The eukaryotic Structural Maintenance of Chromosomes (SMC) family includes the protein complexes cohesin, condensin and Smc5/6. The Smc5/6 complex plays an essential role in the resolution of recombination intermediates formed during mitosis or meiosis, or as a result of the cellular response to replication stress. The Smc5/6 complex has roles in the processes of DNA replication and DNA damage repair; the complex acting to suppress / prevent formation of inappropriate structures that can form during homologous recombination-mediated rescue of replication forks that have stalled (or collapsed) on encountering replication ‘road-blocks’ or obstacles. As well as containing subunits that provide both ubiquitin and SUMO E3-ligase activity (through Nse1 and Nse2 respectively), Smc5/6 is further differentiated from the cohesin and condensin complexes by the fact that the two non-SMC proteins (Nse1 and Nse3) that bind to its kleisin subunit (Nse4) belong to the ‘KITE’ family (kleisin-interacting tandem winged-helix element; 15) rather than the distinct and structurally unrelated ‘HAWK’ family (HEAT proteins associated with kleisins; 16).

Here, we report the cryogenic EM (cryo-EM) structure of the six-subunit budding yeast Smc5/6 holo-complex, reconstituted from recombinant proteins expressed in insect cells – providing both an architectural overview of the entire complex and an understanding of how the Nse1/3/4 subcomplex binds to the hetero-dimeric SMC protein core. Here, we have determined a cryo-EM structure for the budding yeast Smc5/6 ‘holo-complex’, in its apo or non-liganded form. Our study serves to confirm the overall architecture of the complex, plus provide details of how and where the Nse1/Nse3/Nse4 KITE-kleisin subcomplex interacts with the Smc5/Smc6/Nse2 core. Additional experiments also reveal the presence of a crucial interface formed between the head domain of Smc5 and Nse1, which utilises the equivalent of the ‘W-loop’ or ‘F-loop’ found in Smc4 and Smc1 respectively. Notably, mutations that alter the surface-charge profile of the region of Nse1 which accepts the Smc5-loop, lead to a slow-growth phenotype and a global reduction in the chromatin-associated fraction of the Smc5/6 complex, as judged by single molecule localisation microscopy experiments in live yeast. Taken together, our data uncover an unanticipated degree of functional equivalence between KITE and HAWK accessory subunits.

> MTSLIDLGRYVERTHHGEDTEPRSKRVKIAKPDLSSFQPGSIIKIRLQDFVTYTLTEFNLSPSLNMIIGPNGSGKSTFVCAVCLGLAGKPEYIGRSKKVEDFIKNGQDVSKIEITLKNSPNVTDIEYIDARDETIKITRIITRSKRRSDYLINDYQVSESVVKTLVAQLNIQLDNLCQFLSQERVEEFARLKSVKLLVETIRSIDASLLDVLDELRELQGNEQSLQKDLDFKKAKIVHLRQESDKLRKSVESLRDFQNKKGEIELHSQLLPYVKVKDHKEKLNIYKEEYERAKANLRAILKDKKPFANTKKTLENQVEELTEKCSLKTDEFLKAKEKINEIFEKLNTIRDEVIKKKNQNEYYRGRTKKLQATIISTKEDFLRSQEILAQTHLPEKSVFEDIDIKRKEIINKEGEIRDLISEIDAKANAINHEMRSIQRQAESKTKSLTTTDKIGILNQDQDLKEVRDAVLMVREHPEMKDKILEPPIMTVSAINAQFAAYLAQCVDYNTSKALTVVDSDSYKLFANPILDKFKVNLRELSSADTTPPVPAETVRDLGFEGYLSDFITGDKRVMKMLCQTSKIHTIPVSRRELTPAQIKKLITPRPNGKILFKRIIHGNRLVDIKQSAYGSKQVFPTDVSIKQTNFYQGSIMSNEQKIRIENEIINLKNEYNDRKSTLDALSNQKSGYRHELSELASKNDDINREAHQLNEIRKKYTMRKSTIETLREKLDQLKREARKDVSQKIKDIDDQIQQLLLKQRHLLSKMASSMKSLKNCQKELISTQILQFEAQNMDVSMNDVIGFFNEREADLKSQYEDKKKFVKEMRDTPEFQSWMREIRSYDQDTKEKLNKVAEKYEEEGNFNLSFVQDVLDKLESEIAMVNHDESAVTILDQVTAELRELEHTVPQQSKDLETIKAKLKEDHAVLEPKLDDIVSKISARFARLFNNVGSAGAVRLEKPKDYAEWKIEIMVKFRDNAPLKKLDSHTQSGGERAVSTVLYMIALQEFTSAPFRVVDQINQGMDSRNERIVHKAMVENACAENTSQYFLITPKLLTGLHYHEKMRIHCVMAGSWIPNPSEDPKMIHFGETSNYSFD;> MISTTISGKRPIEQVDDELLSLTAQQENEEQQQQRKRRRHQFAPMTQFNSNTLDEDSGFRSSSDVATADQDNFLEESPSGYIKKVILRNFMCHEHFELELGSRLNFIVGNNGSGKSAILTAITIGLGAKASETNRGSSLKDLIREGCYSAKIILHLDNSKYGAYQQGIFGNEIIVERIIKRDGPASFSLRSENGKEISNKKKDIQTVVDYFSVPVSNPMCFLSQDAARSFLTASTSQDKYSHFMKGTLLQEITENLLYASAIHDSAQENMALHLENLKSLKAEYEDAKKLLRELNQTSDLNERKMLLQAKSLWIDVAHNTDACKNLENEISGIQQKVDEVTEKIRNRQEKIERYTSDGTTIEAQIDAKVIYVNEKDSEHQNARELLRDVKSRFEKEKSNQAEAQSNIDQGRKKVDALNKTIAHLEEELTKEMGGDKDQMRQELEQLEKANEKLREVNNSLVVSLQDVKNEERDIQHERESELRTISRSIQNKKVELQNIAKGNDTFLMNFDRNMDRLLRTIEQRKNEFETPAIGPLGSLVTIRKGFEKWTRSIQRAISSSLNAFVVSNPKDNRLFRDIMRSCGIRSNIPIVTYCLSQFDYSKGRAHGNYPTIVDALEFSKPEIECLFVDLSRIERIVLIEDKNEARNFLQRNPVNVNMALSLRDRRSGFQLSGGYRLDTVTYQDKIRLKVNSSSDNGTQYLKDLIEQETKELQNIRDRYEEKLSEVRSRLKEIDGRLKSTKNEMRKTNFRMTELKMNVGKVVDTGILNSKINERKNQEQAIASYEAAKEELGLKIEQIAQEAQPIKEQYDSTKLALVEAQDELQQLKEDINSRQSKIQKYKDDTIYYEDKKKVYLENIKKIEVNVAALKEGIQRQIQNACAFCSKERIENVDLPDTQEEIKRELDKVSRMIQKAEKSLGLSQEEVIALFEKCRNKYKEGQKKYMEIDEALNRLHNSLKARDQNYKNAEKGTCFDADMDFRASLKVRKFSGNLSFIKDTKSLEIYILTTNDEKARNVDTLSGGEKSFSQMALLLATWKPMRSRIIALDQFDVFMDQVNRKIGTTLIVKKLKDIARTQTIIITPQDIGKIADIDSSGVSIHRMRDPERQNNSNFYN;> MGSYPYDVPDYAGSGALNDNPIPKSVPLHPKSGKYFHNLHARDLSNIYQQCYKQIDETINQLVDSTSPSTIGIEEQVADITSTYKLLSTYESESNSFDEHIKDLKKNFKQSSDACPQIDLSTWDKYRTGELTAPKLSELYLNMPTPEPATMVNNTDTLKILKVLPYIWNDPTCVIPDLQNPADEDDLQIEGGKIELTCPITCKPYEAPLISRKCNHVFDRDGIQNYLQGYTTRDCPQAACSQVVSMRDFVRDPIMELRCKIAKMKESQEQDKRSSQAIDVL;> MGSSHHHHHHSSGRENLYFQGHMEVHEEQVSAPVTGDATAKYLLQYILSARGICHENALILALMRLETDASTLNTEWSIQQWVDKLNDYINAINVKLNLLGYKIIRINHGIGRNAVTLKAKQNFESFEDNTAIRAHNNDYAVLQSIVLPESNRFFVYVNLASTEETKLATRFNQNEIEFMKWAIEQFMISGETIVEGPALETSIIVKEVNRILVAATGDSNLAKWRKFSTFTVGSTNLFQFQELTATDIEDLLLRLCELKWFYRTQEGKFGIDLRCIAELEEYLTSMYNLNTCQNCHKLAIQGVRCGNESCREENEETGENSLSQIWHVDCFKHYITHVSKNCDRCGSSLITEGVYVI;> MSSIDNDSDVDLTEDLAVAKIVKENPVARKMVRYILSRGESQNSIITRNKLQSVIHEAAREENIAKPSFSKMFMDINAILYNVYGFELQGLPSKNNMNAGGNGSNSNTNKSMPEPLGHRAQKFILLNNVPHSKNFDDFKILQSAHTYEELIVTGEYIGDDIASGTSNTLESKLSTDRDLVYKGVLSVILCIVFFSKNNILHQELIKFLETFGIPSDGSKIAILNITIEDLIKSLEKREYIVRLEEKSDTDGEVISYRIGRRTQAELGLESLEKLVQEIMGLEKEQTKSLHDDIIKSIGDSYSI;> MSSTVISRKRRNSTVTEPDSSGETRKQKKSRSDEKSSSSKDGDPQLEFKVLQGYRDLESEMHKGRAQVTRTGDIGVAMDNLNAVDSLFNKVIGIKNNGLFAHDARAMVSISELAQISVRNLKFDDSRSMVNLENIVNSLKRYMLKEHFKLNNIAENRNDLTLAADEQSAADQQEESDGDIDRTPDDNHTDKATSSFKATSMRHSYLQQFSHYNEFSQFNWFRIGALYNTISKNAPITDHLMGPLSIEKKPRVLTQRRRNNDQVGEKITAEKITQHSLNSTQQETTPEQVKKCFKKLSKKLGPEGSINLFKFIIDPNSFSRSIENLFYTSFLIKEGKLLMEHDEEGLPTIKIKQSISHTDSRSKEIERQRRRAAHQNHIIFQMDMPTWRKLIKKYNITSPFLDGSSGMAEIGTGFPFDPHYVEVLGERMHYVDVGPRDGTPVLFLHGNPTSSYVWRNIIPHVAPTHRCIAPDLIGMGKSDKPDLGYFFDDHVRFMDAFIEALGLEEVVLVIHDWGSALGFHWAKRNPERVKGIAFMEFIRPIPTWDEWPEFARETFQAFRTTDVGRKLIIDQNVFIEGTLPMGVVRPLTEVEMDHYREPFLNPVDREPLWRFPNELPIAGEPANIVALVEEYMDWLHQSPVPKLLFWGTPGVLIPPAEAARLAKSLPNCKAVDIGPGLNLLQEDNPDLIGSEIARWLSTLEISGGSEQKLISEEDL>DNTVRVGVSRNTSGAAGQTLFRNFYLLRCNILADGRNATKAVQSHFPFLSRAVRCLSPLAAHCADRTLRRDNVKQILTRELPFSSDLINYAHHVNSSSLTTSQGVEAARLVAQVYGEQVPFDHIYPTGSATYCPGAIANAISRIMAGFVPREGDDFAPSGPIDYLAADLIAYKFVLPYMLDMVDGRPQIVLPSHTVEEMLTNTSLLNSIDASFGIEARSDQRMTRDAAEMSSRSLNELEDHDQRGRMPWKIMLGMMAAQLKVELDALADERTESQANAHVTSFGSRLFNQMSAFVTIDHEL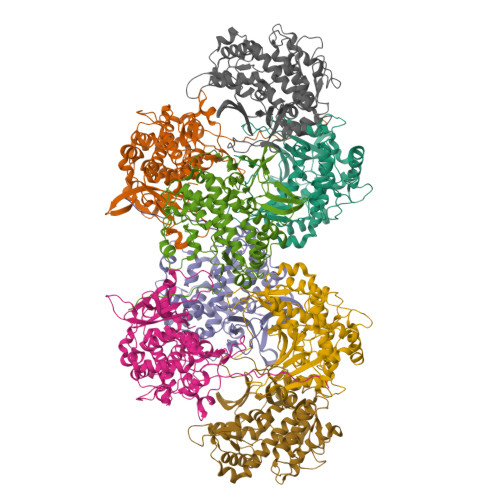MELALLIKEQGFAMNPGQIASKWSLIRRSGPTRPLSGARLEIRNGNWMIREGDQTLLSVSPARMA[8x]> SNAEDSTPTPADSGSPSPPPAASGGTSDGSAASPITSPTTAGAATPASSASGEPIRIGVLLTLSGPQGVNGEGNLRGLTLALDQAGMQFGGRPVELIIEDSAGQPEQAITKTRQLIERDRVHLIAGITLSNEAAAVRDILVQAEMPTIVTNAGLQALTRDPAMRSPYLFRVSFANGQYDAPAADYAYETLGYRRMVLHAADYAAGHEEMAAFRSRFEQAGGEIVDEVVAPIGTQDFGPYLQRIEQAAAEADAVFAFHGTSTDAIRFLVQYQEFGLKDSIPLIPSGADVDQSILPEIGDAALGLVSGTLYTAYNDTPESQEFVEAFTARHEGILPGLVDYAGYIGGRVIAEALTAIDGEVENKEALLEALKAVEF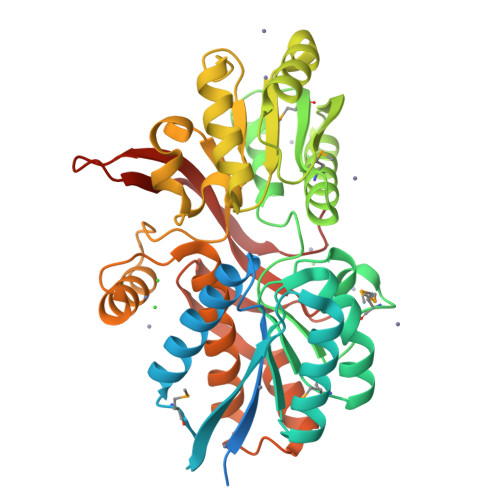TGPAGNFRFHPESQGPVTTILLCRVEQLDDGTYANIVVDRIPDFDDLSF> DYKDDDDKSLEVLFQGPMDVDAEREKITQEIKELERILDPGSSGSHVEISESSLESDSEADSLPSEDLDPADPPISEEERWGEASNDEDDPKDKTLPEDPETCLQLNMVYQEVIQEKLAEANLLLAQNREQQEEL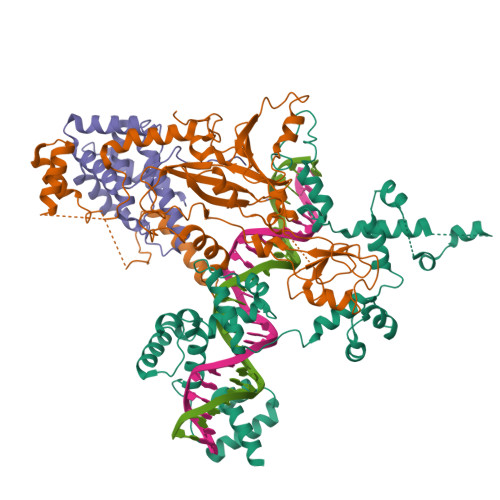MRDLAGSKGTKVKDGKSLPPSTYMGHFMKPYFKDKVTGVGPPANEDTREKAAQGIKAFEELLVTKWKNWEKALLRKSVVSDRLQRLLQPKLLKLEYLHQKQSKVSSELERQALEKQGREAEKEIQDINQLPEEALLGNRLDSHDWEKISNINFEGSRSAEEIRKFWQNSEHPSINKQEWSREEEERLQAIAAAHGHLEWQKIAEELGTSRSAFQCLQKFQQHNKALKRKEWTEEEDRMLTQLVQEMRVGSHIPYRRIVYYMEGRDSMQLIYRWTKSLDPGLKKGYWAPEEDAKLLQAVAKYGEQDWFKIREEVPGRSDAQCRDRYLRRLHFSLKKGRWNLKEEEQLIELIEKYGVGHWAKIASELPHRSGSQCLSKWKIMMGKKQGL;> MAEGSRGGPTCSGVGGRQDPVSGSGGCNFPEYELPELNTRAFHVGAFGELWRGRLRGAGDLSLREPPASALPGSQAADSDREDAAVARDLDCSLEAAAELRAVCGLDKLKCLEDGEDPEVIPENTDLVTLGVRKRFLEHREETITIDRACRQETFVYEMESHAIGKKPENSADMIEEGELILSVNILYPVIFHKHKEHKPYQTMLVLGSQKLTQLRDSIRCVSDLQIGGEFSNTPDQAPEHISKDLYKSAFFYFEGTFYNDKRYPECRDLSRTIIEWSESHDRGYGKFQTARMEDFTFNDLCIKLGFPYLYCHQGDCEHVIVITDIRLVHHDDCLDRTLYPLLIKKHWLWTRKCFVCKMYTARWVTNNDSFAPEDPCFFCDVCFRMLHYDSEGNKLGEFLAYPYVDPGTFN;> HHHHHHSENLYFQGMGTPPGLQTDCEALLSRFQETDSVRFEDFTELWRNMKFGTIFCGRMRNLEKNMFTKEALALAWRYFLPPYTFQIRVGALYLLYGLYNTQLCQPKQKIRVALKDWDEVLKFQQDLVNAQHFDAAYIFRKLRLDRAFHFTAMPKLLSYRMKKKIHRAEVTEEFKDPSDRVMKLITSDVLEEMLNVHDHYQNMKHVISVDKSKPDKALSLIKDDFFDNIKNIVLEHQQWHKDRKNPSLKSKTNDGEEKMEGNSQETERCERAESLAKIKSK>[2x]MDASTLGSFTGGQLRRLGSVAGLSRADVETYAQVLTDALGPVAQRPLSLAPPTRTFLS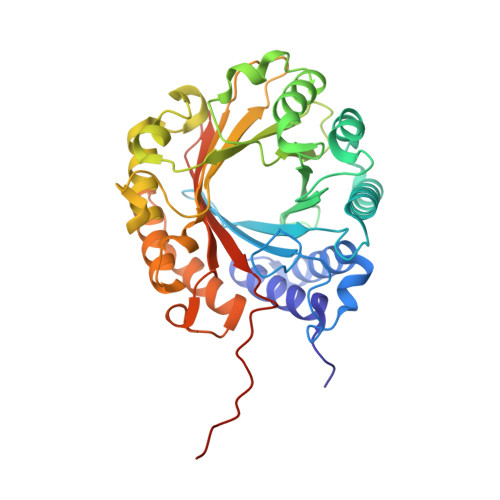DDHTPVEFSLSFRPGAAPAMRVLVEPGCGATSLADNGRAGLEAVRTMARRWHFTTDALDELLDLFLPPAPQGPLALWCALELRPGGVPGVKVYLNPAVGGEERSAATVREALRRLGHHQAFDSLPQGSGYPFLALDLGNWTEPRAKVYLRHDNLTAGRAARLSRTDSGLVPTAVEGFFRTAAGPGSDAGGLDGRPAQSCHSFTDPGAERPSGFTLYIPVRDYVRHDGEALARASTVLHHHGMDASVLHRALAALTERRPEDGVGLIAYLALAGQRDQPPRVTAYLSSEAYTVRPPVVELVPRGSHHHHHHHH> GSPSRRNF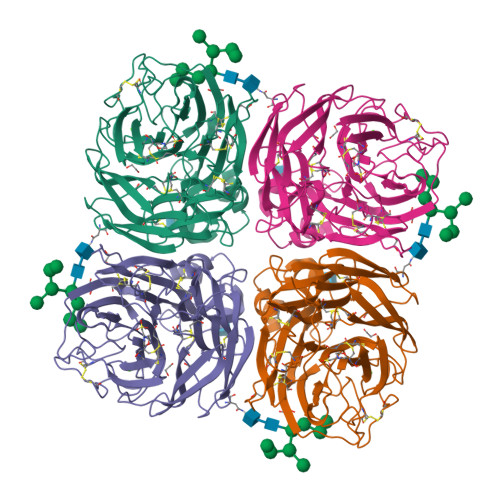NNLTKGLCTINSWHIYGKDNAVRIGESSDVLVTREPYVSCDPDECRFYALSQGTTIRGKHSNGTIHDRSQYRALISWPLSSPPTVHNSRVECIGWSSTSCHDGKSRMSICISGPNNNASAVVWYNRRPVAEINTWARNILRTQESECVCHNGVCPVVFTDGSATGPADTRIYYFKEGKILKWESLTGTAKHIEECSCYGERTGITCTCRDNWQGSNRPVIQIDPVAMTHTSQYICSPVLTDNPRPNDPNIGKCNDPYPGNNNNGVKGFSYLDGANTWLGRTISTASRSGYEMLKVPNALTDDRSKPIQGQTIVLNADWSGYSGSFMDYWAEGDCYRACFYVELIRGRPKEDKVWWTSNSIVSMCSSTEFLGQWNWPDGAKIEYFL>[4x]MARIAQHISELIGGTPLVRLNSVVPDGAGTVAAKVEYLNPGGSSKDRIAVKMIEAAEASGQLKPGGTIVEPTSGNTGVGLALVAQRRGYKCVFVCPDKVSEDKRNVLIAYGAEVVVCPTAVPPHDPASYYSVSDRLVRDIDGAWKP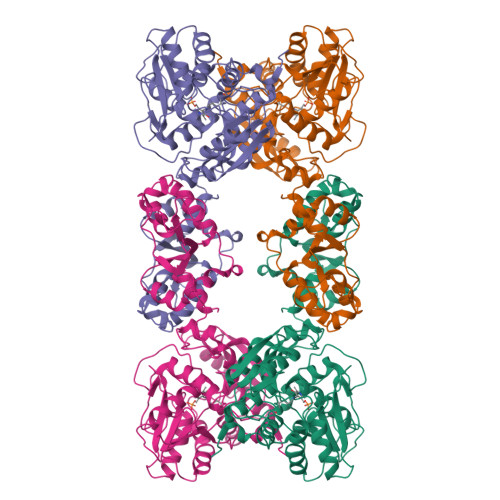DQYANPEGPASHYVTTGPEIWADTEGKVTHFVAGIGTGGTITGAGRYLKEVSGGRVRIVGADPEGSVYSGGAGRPYLVEGVGEDFWPAAYDPSVPDEIIAVSDSDSFDMTRRLAREEAMLVGGSCGMAVVAALKVAEEAGPDALIVVLLPDGGRGYMSKIFNDAWMSSYGFLRSRLDGSTEQSTVGDVLRRKSGALPALVHTHPSETVRDAIGILREYGVSQMPVVGAEPPVMAGEVAGSVSERELLSAVFEGRAKLADAVSAHMSPPLRMIGAGELVSAAGKALRDWDALMVVEEGKPVGVITRYDLLGFLSEGAGRRKLAAALEHHHHHH5-(aminomethyl)-2-methoxyphenol | C8 H11 N O2 | 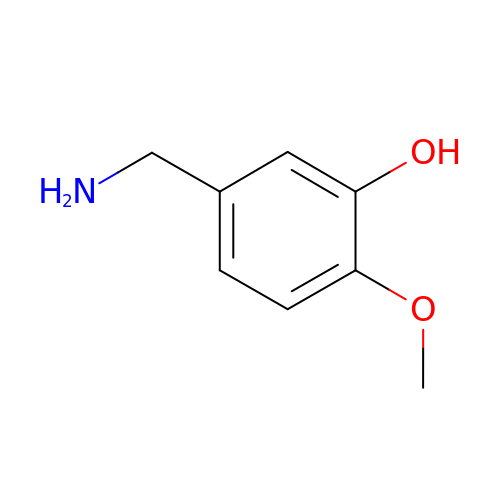HJIDMVZCXORAIG-UHFFFAOYSA-N> IPGANLLRMAFGVIGTQIVRYRKFEQRVKNDQAQYVSMFGEPFDLAASVQRVRRDQ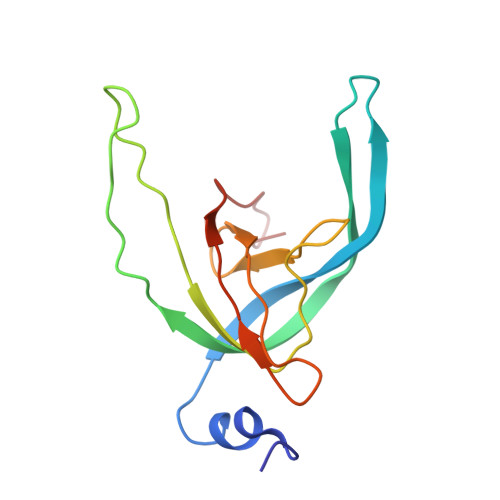YAQFNLEFQRNYVMIFANFDMVDLDRNMAGDQFLWTGRVFQLESQGSWFYQDGWGVCLAVDIGAAKA>GDGAGASRQRKLEALIRDPRSPINVESLLDGLNSLVLDLDFPALRKNKNIDNFLNRYEKIVKKIRGLQMKAEDYDVVKVIGRGAFGEVQLVRHKASQKVYAMKLLSKFEMIKRSDSAFFWEERDIMAFANSPWVVQLFYAFQDDRYLYMVMEYMPGGDLVNLMSNYDVPEKWAKFYTAEVVLALDAIHSMGLIHRDVKPDNMLLDKHGHLKLADFGTCMKMDETGMVHCDTAVGTPDYISPEVLKSQGGDGFYGRECDWWSVGVFLYEMLVGDTPFYADSLVGTYSKIMDHKNSLCFPEDAEISKHAKNLICAFLTDREVRLGRNGV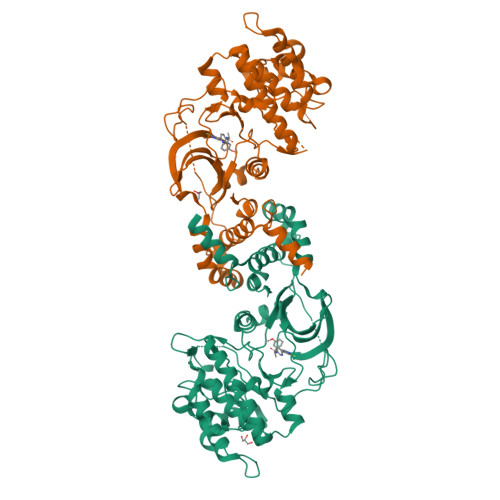EEIRQHPFFKNDQWHWDNIRETAAPVVPELSSDIDSSNFDDIEDDKGDVETFPIPKAFVGNQLPFIGFTYYR[8x]>[6x]KLTKEELKEIVTMMVNKLTNRLSEQNINIIVTDKAKDKIAEEGYDPEYGARPLIRAIQKTIEDNLSELILDGNQIEGKKVTV;>LTKINETESEKLLSLEDTLHERVIGQKDAVNSISKAVRRARAGLKDPKRPIGSFIFLGPTGVGKTELARALAESMFGDDDAMIRVDMSEFMEKHAVSRLVGAPPGYVGHDDGGQLTEKVRRKPYSVILFDEIEKAHPDVFNILLQVLDDGHLTDTKGRTVDFRNTIIIMTSNVGAQELQDQRFAGFGGSSDGQDYETIRKTMLKELKNSFRPEFLNRVDDIIVFH[6x];>NNLKEIEQEIEKVKNEKDAAVHAQEFENAANLRDKQTKLEKQYEEAKNEWKNAQN[6x];>SVVDTVAILKGLRDRYEAHHRINISDEAIEAAVKLSNRYVSDRFLPDKAIDLIDEASSKVRLKSHTTPNNLKEIEQEIEKVKNEKDAAVHAQEFENAANLRDKQTKLEKQYEEAKNEWKNAQNG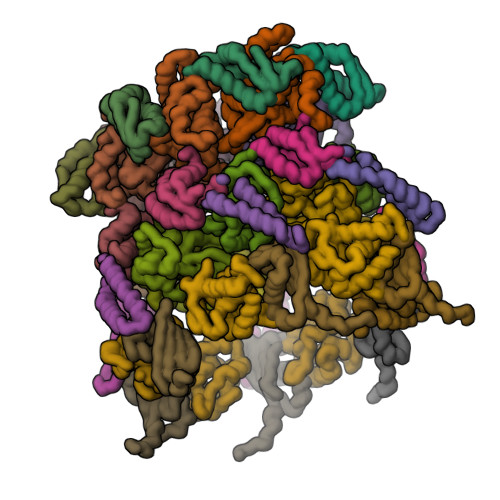MSTSLSEEDIAEVIAGWTGIP[6x];>[6x]TLDSLARDLTVIAKDGTLDPVIGRDKEITRVIEVLSRRTKNNPVLIGEPGVGKTAIAEGLAQAIVNNEVPETLKDKRVMSLDMGTVVAGTKYRGEFEERLKKVMEEIQQAGNVILFIDELHTLVGAGGAEGAIDASNILKPALARGELQCIGATTLDEYRKNIEKDAALERRFQPVQVDEP;>RLTERAQRVLAHAQEEAIRLNHSNIGTEHLLLGLMKEPEGIAAKVLESFNITEDKVIEEVEKLIGHGQDHVGTLHYTPRAKKVIELSMDEARKLHHNFVGTEHILLGLIRENEGVAARVFANLDLNITKARAQVVKALGNPEMSNKNAQASKSNNTP[6x];>MRIERVDDTTVKLFITYSDIEARGFSREDLWTNRKRGEEFFWSMMDEINEEEDFVVEGPLWIQVHAFEKGVEVTISKSKNEDMMNMSDDD[6x]>MPFTIDSARGIFPNTLAADVVPATIARFSQLNAEDQLALIWFASLEMGKTLTIAAPGAASMQLAENALKEIQAMGPLQQTQAMCDLANRADTPLCRTYASWSPNIKLGFWYRLGELMEQGFVAPIPAGYQLSANANAVLATIQGLESGQQITVLRNAVVDMGFTAGKDGKRIAEPVVPPQDTASRTKVSIEGVTNATVLNYMDNLNANDFDTLIELFTSDGALQPPFQRPIVGKENVLRFFREECQNLKLIPERGVTEPAEDGFTQIKVTGKVQTPWFGGNVGMNIA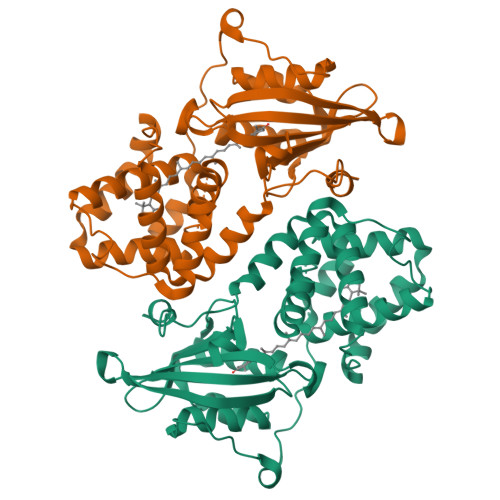WRFLLNPEGKIFFVAIDLLASPKELLNFAVHHHHHH[2x]>MDWGRFVEEKVREIRETVGDSKAIIALSGGVDSSTAAVLAHKAIGDRLHAVFVNTGFLRKGEPEFVVKTFRDEFGMNLHYVDAQDRFFSALKGVTDPEEKRKIIGRVFIEVFEEVAKKIGAEYLIQGTIAPDWIESQGKIKSHHNVGGL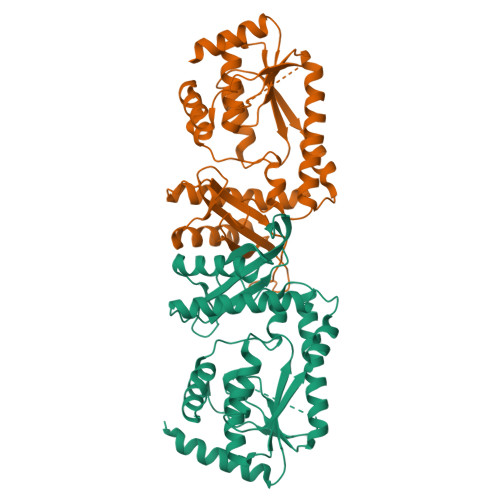PEKLNLKLIEPLRDLYKDEVRELAKFLGLPEKIYNRMPFPGPGLAVRVIGEVTPEKIRIVREANAIVEEEVERAGLRPWQAFAVLLGVKTVGVQGDIRAYKETIAVRIVESIDGMTANAMNVPWEVLQRIAFRITSEIPEVGRVLYDITNKPPATIEFE[2x]6-chloranyl-3-[3-[(1~{S})-1-(4-chlorophenyl)ethyl]-5-phenyl-imidazol-4-yl]-~{N}-[2-(4-cyclohexylpiperazin-1-yl)ethyl]-1~{H}-indole-2-carboxamide | C38 H42 Cl2 N6 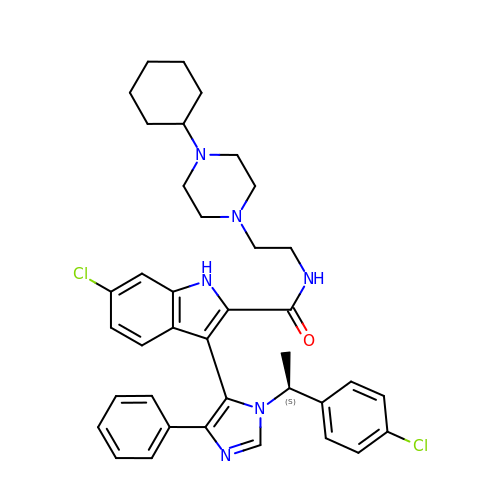O | NPCLCDAMEOOZHU-SANMLTNESA-N1-[(2S)-2-methyl-3-sulfanyl-propanoyl]piperidine-4-carboxylic acid | C10 H17 N O3 S | 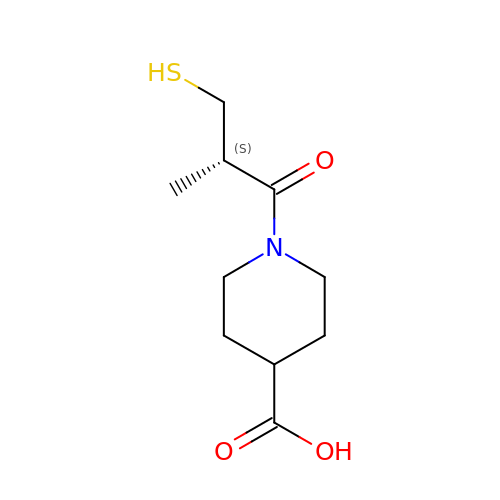VYYKYNRWNVSARB-SSDOTTSWSA-N>[2x]MKLNKQNLTQLAPEVKLPAYTLADTRQGIAHIGVGGFHRAHQAYYTDALMNTGEGLDWSICGVGLRSEDRKARDDLAGQDYLFTLYELGDTDDTEVRVIGSISDMLLAEDSAQALIDKLASPEIRIVSLTITEGGYCIDDSNGEFMAHLPQIQHDLAHPSSPKTVFGFIC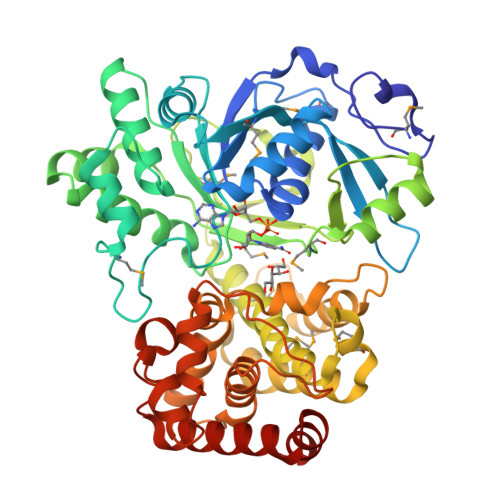AALTQRRAAGIPAFTVMSCDNLPHNGAVTRKALLAFAALHNAELHDWIKAHVSFPNAMVDRITPMTSTAHRLQLHDEHGIDDAWPVVCEPFVQWVLEDKFVNGRPAWEKVGVQFTDDVTPYEEMKIGLLNGSHLALTYLGFLKGYRFVHETMNDPLFVAYMRAYMDLDVTPNLAPVPGIDLTDYKQTLVDRFSNQAIADQLERVCSDGSSKFPKFTVPTINRLIADGRETERAALVVAAWALYLKGVDENGVSYTIPDPRAEFCQGLVSDDALISQRLLAVEEIFGTAIPNSPEFVAAFERCYGSLRDNGVTTTLKHLLKKPV>[2x]MGSSHHHHHHSNGSMNSDQVTLVGQVFESYVSEYHKNDILLILKERDEDAHYPVVVNAMTLFETNMEI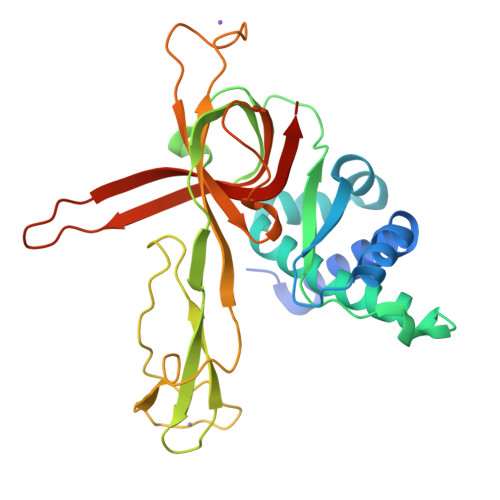GEYFNMFPSEVLTIFDSALRRSALTILQSLSQPEAVSMKQNLHARISGLPVCPELVREHIPKTKDVGHFLSVTGTVIRTSLVKVLEFERDYMCNKCKHVFVIKADFEQYYTFCPPSSCPSLESCDSSKFTCLSGLSSSPTRCRDYQEIKIQEQVQRLSVGSIPRSMKVILEDDLVDSCKSGDDLTIYGIVMQRWKPFQQDVRAEVEIVLKANYIQVNNEQSSG>SVDDSKYQCVKLNDGHFMPVLGFGTYAPAEVPKSKALEAVKLAIEAGFHHIDSAHVYNNEEQVGLAIRSKIADGSVKREDIFYTSKLWSNSHRPELVRPALERSLKNLQLDYVDLYLIHFPVSVKPGEEVIPKDENGKILFDTVDLCATWEAMEKCKDAGLAKSIGVSNFNHRLLEMILNKPGLKYKPVCNQVECHPYFNQRKLLDFCKSKDIVLVAYSALGSHREEPWVDPNSPVLLEDPVLCALAKKHKRTPALIALRYQLQRGVVVLAKSYN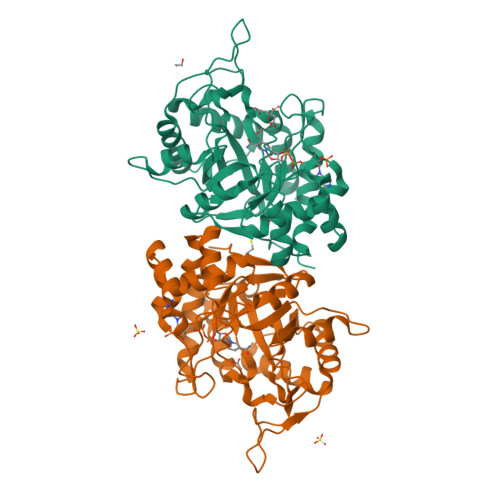EQRIRQNVQVFEFQLTSEEMKAIDGLNRNVRYLTLDIFAGPPNYPFSDEY[2x]>MGRLRRRQEIIDHEEEESNDDVSSRRGKLSLAETFRWLDSSEHRRIETDGHNDYKYIIHPKNRWYKAWEMFILVWAIYSSLFTPMEFGFFRGLPERLFVLDIVGQIAFLVDIVLQFFVAYRDTQTYRTVYKPTRIAFRYLKSHFLMDFIGCFPWDLIYKASGKHELVRYLLWIRLFRVRKVVEFFQRLEKDTRINYLFTRILKLLFVEVYCTHTAACIFYYLATTLPPENEGYTWIGSLKLGDYSYENFREIDLWKRYTTALYFAIVTMATVGYGDIHAVNLREMIFV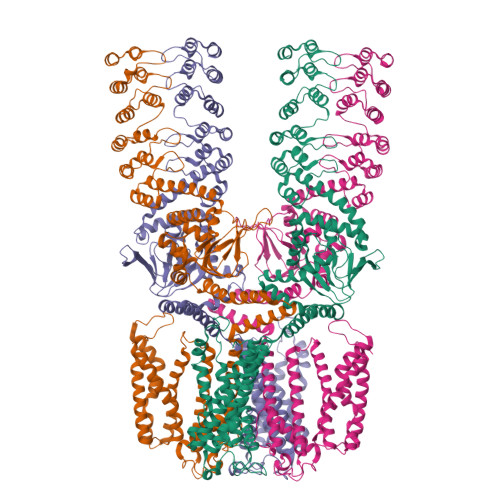MIYVSFDMVLGAYLIGNITALIVKGSNTERFRDKMNDLISFMNRKKLGRDLRSQITGHVRLQYDSHYTDTVMLQDIPASIRAKIAQLLYLPYIKKVPLFKGCSTEFINQIVIRLHEEYFLPGEVITEQGNVVDHLYFVCEGLLEALVTKTDGSEESVTLLGPHTSFGDISIICNISQPFTVRVCELCHLLRLDKQSFSNILEIYFHDGRTILNNIMEEKESNDRIKKLESDIVIHIGKQEAELALKVNSAAFQGDFYQLKSLIRSGADPNKTDYDGRSPLHLAACRGYEDITLFLIQEGVDVNLKDKFGHTPLFEAVKAGQEGVIGLLVKEGASFNLEDSGNFLCTTVAKGDSDFLKRLLSSGMNPNSEDYDHRTPLHVAASEGLFLMAKMLVEAGASVISKDRWGNSPLDEARLCGNKKLIKLLEDVKNAQSSIYPSSLRELQEERIERRKCTVFPFHPQEAKEERSRKHGVVVWIPSNLEKLIVTAAKELGLSDGASFVLLSEDQGRITDIDMISDGHKLYMISDTTDQT[4x]>GPGFGGVF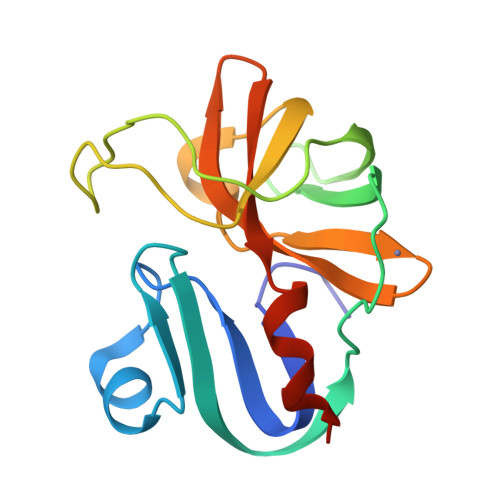VGSFKIINYHLATIEERQSAIYVDWQSDVLVTPIAAHGRHQIARCKCNTGVYYCRHRDKSYPVCFEGPGIQWIEQTEYYPARYQTNVLLAAGPAEAGDCGGLLVCPHGVIGLLTAGGGGIVAFTDIRNLLWLDTDAMEQ[6x]>AHMFMAENRLQLQKGSAEETIERFYNRQGIETIEGFQQMFVTKTLNTEDTDEVKILTIWESEDSFNNWLNSDVFKEAHKNVRLKSD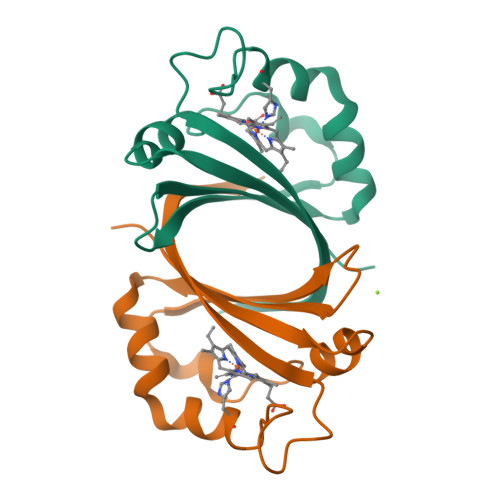DDGQQSPILSNKVFKYDIGYHYQK[2x]N-[6-(4-acryloyl-1,4-diazepan-1-yl)-2-(pyridin-2-yl)pyrimidin-4-yl]-beta-alanine | C20 H24 N6 O3 | 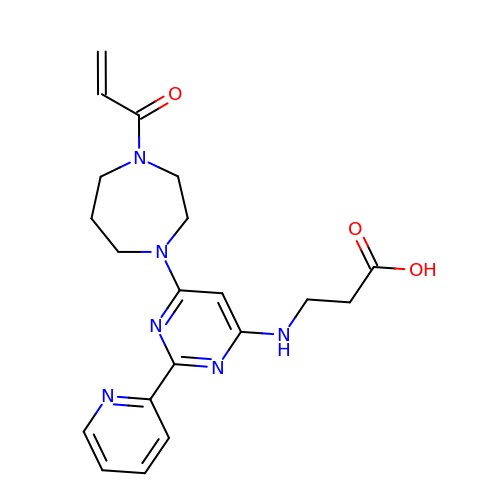GQZPLTPYSQYTFB-UHFFFAOYSA-N> MGGSHHHHHHGMASMSKRITDSQVLGELGETAIKKIVLETGFLYEQRGRLEAGTDGIIELRDPKSGAPLGKLLGVQVKSTESGQYVRENDNSFEYLLKPDDLKYWRTSNIPVIIVLWRKSDETAYWKDVSDCVRGEERRLKFDKGTDVFDPRSADRIGALTIDRRTPGVFLPPLNKGEDAIINLLRIRLPDEIFISTSPFGSGRDAVPELVKHGNVRFDWVIRKRRFVSFFDPREYGTRAIVDLDQVEAVDTKLIAFNDEQDDLNDTMDLLRRTVERQTATQLSFLRKDRLFHFKAVGVGKSRSYRYMSNVNETS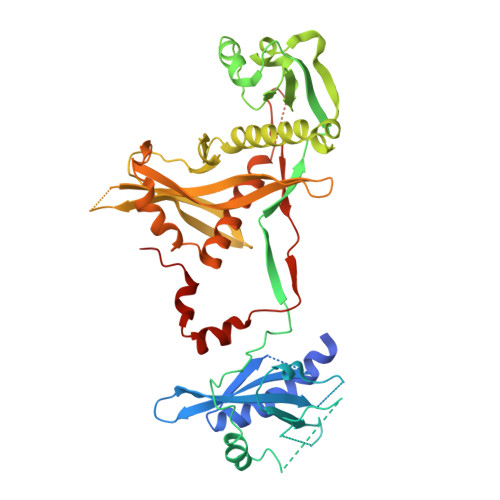AKVVSAYSSKKKDGWGYVRHHAARLRFERLADEWFLVIDPDFHFTTDGFQPHRYPEALLAGKKRLERNAAVRGQVTMWQHLLVESGKHEVGLFDADKPAPLLQFERLPVIQLSQAVPESSWNRTDPRAKEMEAQDLFEEGGVG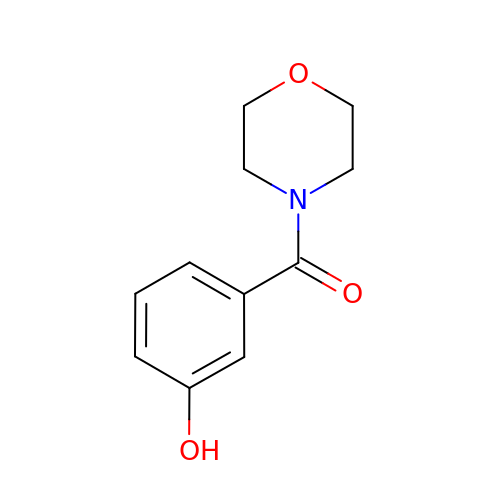(3-hydroxyphenyl)(morpholin-4-yl)methanone | C11 H13 N O3 | PELYAGCBLDBUTI-UHFFFAOYSA-N N-[(3S,4R,5R,6R)-4,5,6-trihydroxyazepan-3-yl]acetamide | C8 H16 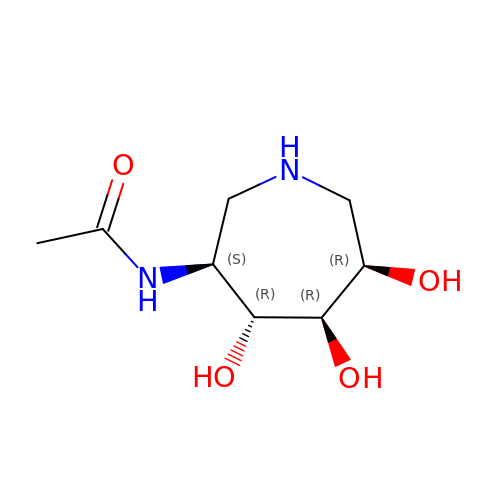N2 O4 | RGHXJBVAPJFIEQ-LXGUWJNJSA-N> MKEFYLTVEQIGDSIFERYIDSNGRERTREVEYKPSLFAHCPESQATKYFDIYGKPCTRKLFANMRDASQWIKRMEDIGLEALGMDDFKLAYLSDTYNYEIKYDHTKIRVANFDIEVTSPDGFPEPSQAKHPIDAITHYDSIDDRFYVFDLLNSPYGNVEEWSIEIAAKLQEQGGDEVPSEIIDKIIYMPFDNEKELLMEYLNFWQQKTPVILTGWNVESFAIPYVYNRIKNIFGESTAKRLSPHRKTRVKVIENMYGSREIITLFGISVLDYIDLYKKFSFTNQPSYSLDYISEFELNVGKLKYDGPISKLRESNHQRYISYNIIAVYRVLQIDAKRQFINLSLDMGYYAKIQIQSVFSPIKTWDAIIFNSLKEQNKVIPQGRSHPVQPYPGAFVKEPIPNRYKYVMSFDLTSLYPSIIRQVNISPETIAGTFKVAPLHDYINAVA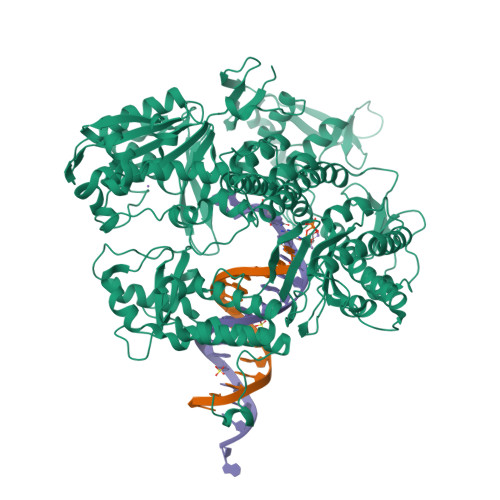ERPSDVYSCSPNGMMYYKDRDGVVPTEITKVFNQRKEHKGYMLAAQRNGEIIKEALHNPNLSVDEPLDVDYRFDFSDEIKEKIKKLSAKSLNEMLFRAQRTEVAGMTAQINRKALINSLYGALGNVWFRYYDLRNATAITTFGQMALQWIERKVNEYLNEVCGTEGEAFVLYGDTDSIYVSADKIIDKVGESKFRDTNHWVDFLDKFARERMEPAIDRGFREMCEYMNNKQHLMFMDREAIAGPPLGSKGIGGFWTGKKRYALNVWDMEGTRYAEPKLKIMGLETQKSSTPKAVQKALKECIRRMLQEGEESLQEYFKEFEKEFRQLNYISIASVSSANNIAKYDVGGFPGPKCPFHIRGILTYNRAIKGNIDAPQVVEGEKVYVLPLREGNPFGDKCIAWPSGTEITDLIKDDVLHWMDYTVLLEKTFIKPLEGFTSAAKLDYEKKASLFDMFDF Vesicle-associated membrane protein 7 (VAMP7), also known as tetanus neurotoxin-insensitive VAMP (TI-VAMP) or synaptobrevin-like 1 (SYBL1), is an R-SNARE that has been implicated in several fusion events, some likely to be in all cells and others occurring at specialized sites in particular types of differentiated cells. VAMP7 and yeast Nyv1p (Wen et al., 2006), along with the yeast and mammalian orthologs of Sec22 (Gonzalez et al., 2001) and Ykt6 (Tochio et al., 2001), comprise the “longin” subfamily of R-SNAREs because they possess a 120–140 residue N-terminal, profilin-like, longin domain (Filippini et al., 2001) that is also found in other proteins including the σ and μ subunits of the AP2 clathrin adaptor complex (Collins et al., 2002) and the SRα subunit of the signal recognition particle receptor. We demonstrate that the clathrin-mediated endocytosis of the SNARE VAMP7 is directly mediated by Hrb, a clathrin adaptor and ArfGAP. Hrb wraps 20 residues of its unstructured C-terminal tail around the folded VAMP7 longin domain, demonstrating that unstructured regions of clathrin adaptors can select cargo.

In order to increase artificially the apparent concentration of the two components and thus make crystallizing a complex of the two more likely, a cDNA encoding the fragment of Hrb mapped as binding VAMP7 longin domain (residues 136–176) was cloned onto the 5′ end of the VAMP7 longin domain cDNA. Following removal of the GST tag, this chimeric construct was crystallized and its structure was determined by SIRAS with a single mercury derivative (Experimental Procedures), because attempts to solve it by molecular replacement using a variety of profilin-like fold proteins as search models failed. The chimeric construct crystallized with four molecules in the asymmetric unit, with the fragments of Hrb binding to each longin domain in an identical manner but with two being intermolecular and two being intramolecular interactions. As expected, the VAMP7 longin domain (residues 1–115) possessed a five-stranded antiparallel β sheet, flanked by helix α1 on one face with helix α2 and a truncated helix α3 on the other. The first 20 residues of the Hrb fragment (residues 136–155) are disordered, and only residues 156–176 are visible in the density. These sit in a hydrophobic groove that wraps halfway around the longin domain and have assumed short stretches of defined secondary structure on binding the longin domain. Residues 156–159 of Hrb form an additional β strand along one edge of VAMP7 longin domain strand β3. The Hrb short β strand then gives way to a single-turn α helix (residues 160–167) that is flanked by proline residues, and contacts the longin domain via hydrophobic interactions using predominantly three leucine residues. Residues 168–176 of Hrb pack against helix α1 of VAMP7 longin domain, with the interaction again being mediated by hydrophobic side chains and also one hydrogen bond between Asn24 of VAMP7 longin domain and Thr170 of Hrb.

>GSVASVHASISGSSASSTSSTPEVKPLKSLLGDSAPTLHLNKGMAILFAVVARGTTILAKHAWCGGNFLEVTEQILAKIPSENNKLTYSHGNYLFHYICQDRIVYLCITDDDFERSRAFSFLNEVKKRFQTTYGSRAQTALPYAMNSEFSSVLAAQLKHHSENHHHHHH[4x]> MAQRVKITTTATPGEIELAFEDTGTGLPVLLVHGFPLDRTMWKAQREELCDEFRVIVPDLRGFGESQVIPGVATMEAMADDLAGLCNHLGLTGKIVLGGLSMGGYVAFAFARKYRDRLAGLILCDTRARPDSPEAKENRRRVAERVRREGPGFIAEEMIPRLCCESTFRNHPEVIEKIRQMILSAPPEGVAAAALGMAERPDSTDLLPALSCPTLVLVGQFDAISP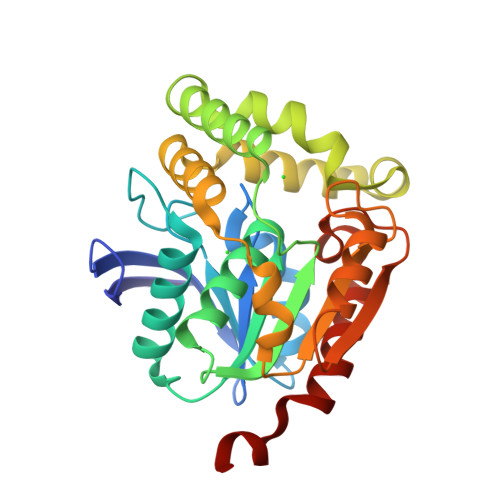PEEMEAMARTIPQSQFVVIPDAGHLPPMEQPERVTQAIREWLRKVHTEAGHHHHHH> MGAEIPKELLRAQTNVILLNV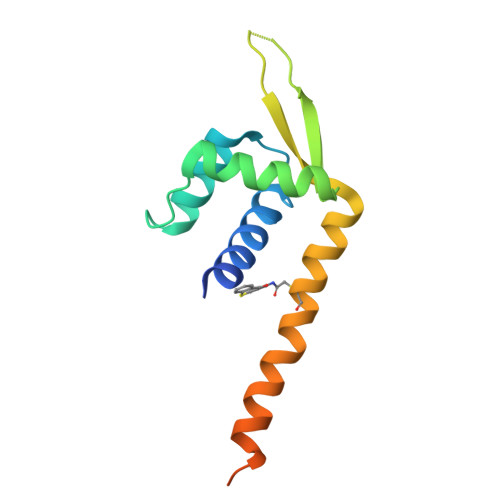LKQGDNYVYGIIKQVKEASNGEMELNEATLYTIFDRLEQDGIISSYWGDESQGGRRKYYRLTEIGHEHMRLACESLSRVDKIIENLEANKKSEAIKSRGGSGGWSHPQFEK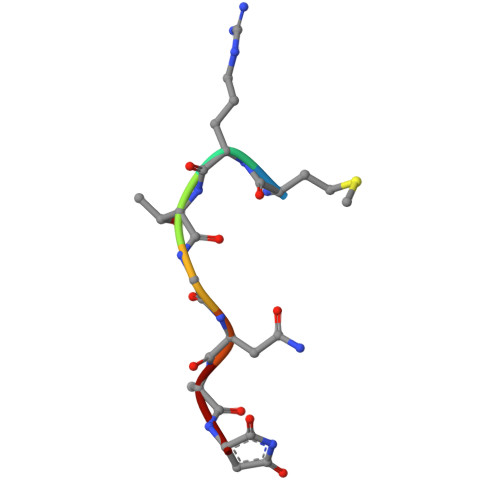> MRTGNAN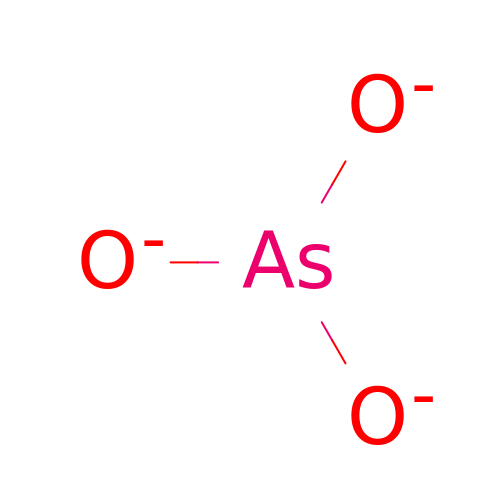ARSENITE | As O3 | OWTFKEBRIAXSMO-UHFFFAOYSA-N> RVEMWNLMPPPAMER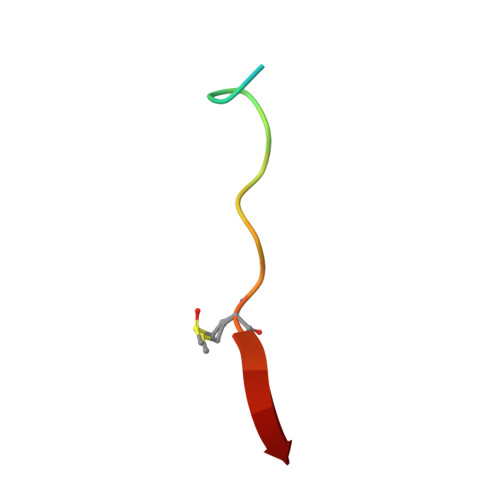LI> LTF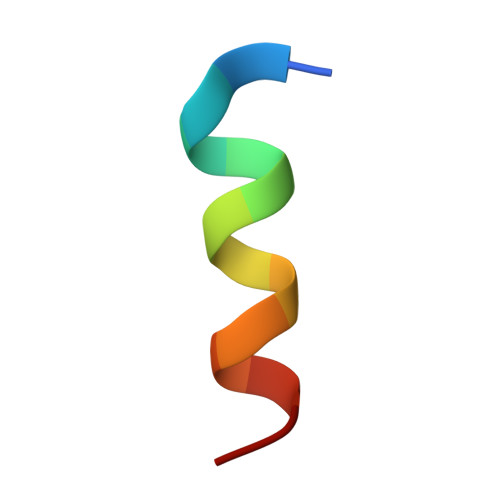DQYWAQLDSAA>[4x]MSLTVKDILDAIQSPDSTPADIAALPLPESYRAITVHKDETEMFAGLETRDKDPRKSIHLDDVPVPELGPGEALVAVMASSVNYNSVHTSI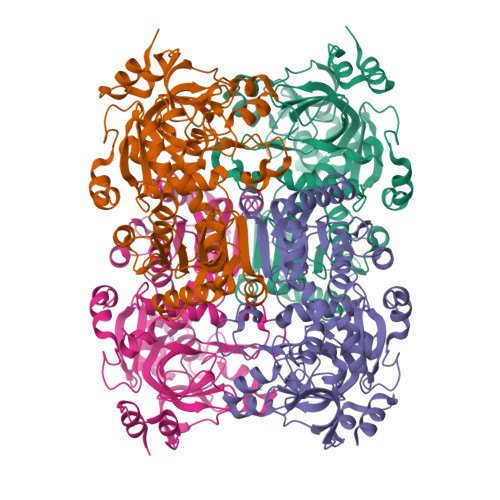FEPLSTFGFLERYGRVSDLAKRHDLPYHVIGSDLAGVVLRTGPGVNAWQAGDEVVAHCLSVELESSDGHNDTMLDPEQRIWGFETNFGGLAEIALVKSNQLMPKPDHLSWEEAAAPGLVNSTAYRQLVSRNGAGMKQGDNVLIWGASGGLGSYATQFALAGGANPICVVSSPQKAEICRAMGAEAIIDRNAEGYRFWKDENTQDPKEWKRFGKRIRELTGGEDIDIVFEHPGRETFGASVFVTRKGGTITTCASTSGYMHEYDNRYLWMSLKRIIGSHFANYREAWEANRLIAKGRIHPTLSKVYSLEDTGQAAYDVHRNLHQGKVGVLCLAPEEGLGVRDREKRAQHLDAINRFRNEGHHHHHH> FDEFPIGDEQDAGILTVAGVYFQPVDMEPAGNSLSKNEADCHMEADISANEKGATLGYGAGDFVPYLHVKAYIQKVGSSKVQEVAFMPMNASDGPHYGANVKFEEGLGKYNIKFEIKAPGNDYLLHVDKETGVTGRFWTEPIVVEWKDFE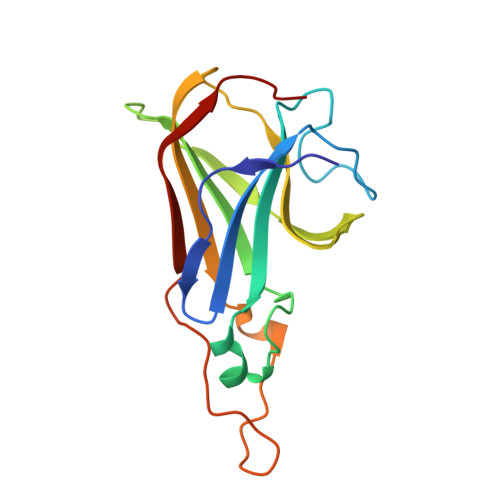WTGPQW>HPE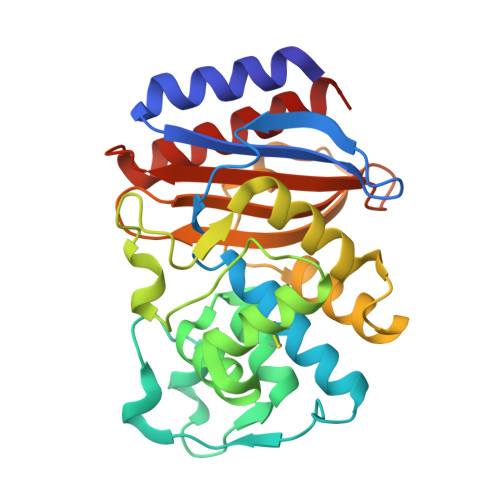TLVKVKDAEDQLGARVGYIELDLNSGKILESFRPEERFPMMSTFKVLLCGAVLSRVDAGQEQLGRRIHYSQNDLVEYSPVTEKHLTDGMTVRELCSAAITMSDNTAANLLLTTIGGPKELTAFLHNMGDHVTRLDRWEPELNEAIPNDERDTTTPAAMATTLRKLLTGELLTLASRQQLIDWMEADKVAGPLLRSALPAGWFIADKSGAGERGSRGIIAALGPDGKPSRIVVIYTTGSQATMDERNRQIAEIGASLIKHW[4x]>[2x]STIPSEIINWTILNEIISMDDDDSDFSKGLIIQFIDQA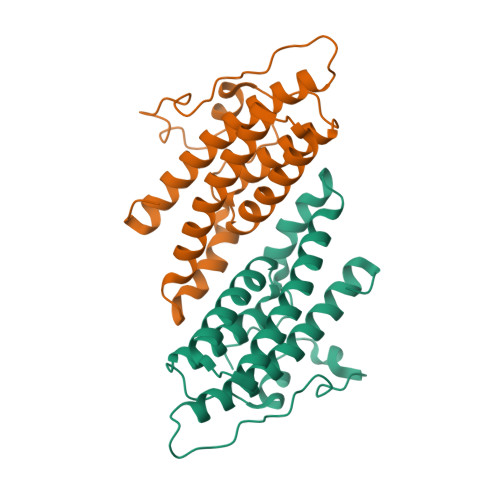QTTFAQMQRQLDGEKNLTELDNLGHFLKGSSAALGLQRIAWVCERIQNLGRKMQHFFPNKTELVNTLSDKSIINGINIDEDDEEIKIQVDDKDENSIYLILIAKALNQSRLEFKLARIELSKYYNTNL>PQSYFNAAAKRQKYAMKPGLSALEKNAVIKAAYRQIFERDITKAYSQSISY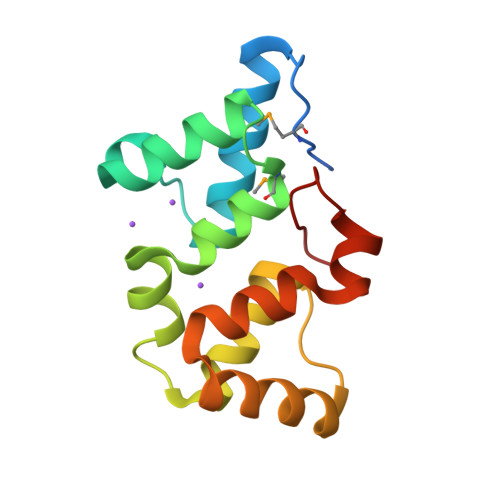LESQVRNGDISMKEFVRRLAKSPLYRKQFFEPFINSRALELAFRHILGRGPSSREEVQKYFSIVSSGGLPALVDALVDSQEYADYFGEETVPYLRG[4x]>[8x]MALVDGFLELERSSGKLEWSAILQKMASDLGFSKILFGLLPKDSQDY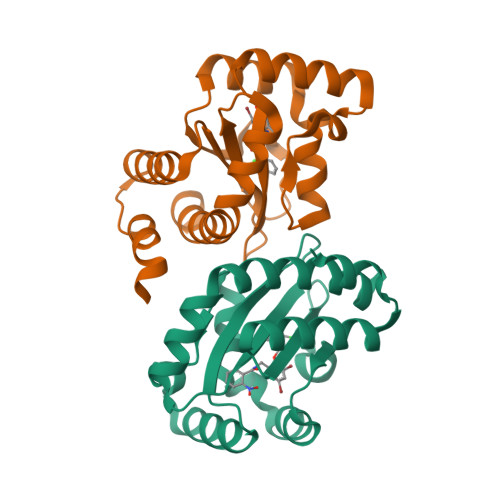ENAFIVGNYPAAWREHYDRAGYARVDPTVSHCTQSVLPIFWEPSIYQTRKQHEFFEEASAAGLVYGLTMPLHGARGELGALSLSVEAENRAEANRFMESVLPTLWMLKDYALQSGAGLAFEHPVSK>LDLFVSPLGRVEGDLDVRVTINDGVVTSAWTEAAMFRGFEIILRGKDPQAGLIVCPRICGICGGSHLYKSAYALDTAWRTHMPPNATLIRNICQACETLQSIPRYFYALFAIDLTNKNYAKSKLYDEAVRRFAPYVGTSYQPGVVLSAKPVEVYAIFGGQWPHSSFMVPGGVMSAPTLSDVTRAIAILEHWNDNWLEKQWLGCSVDRWLENKTWNDVLAWVDENESQYNSDCGFFIRYCLDVGLDKYGQGVGNYLATGTYFEPSLYENPTIEGRNAALIGRSGVFADGRYFEFDQANVTEDVTHSFYEGNRPLHPFEGETIPVNPEDGRRQGKYSWAKSPRYAVPGLGNVPLETGPLARRMA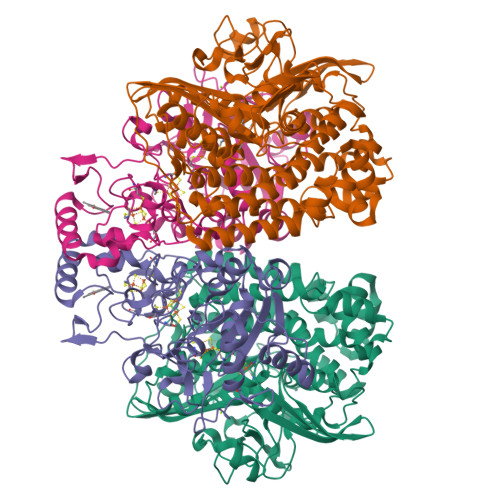ASAPDAETHQDDDPLFADIYNAIGPSVMVRQLARMHEGPKYYKWVRQWLDDLELKESFYTKPVEYAEGKGFGSTEAARGALSDWIVIEDSKIKNYQVVTPTAWNIGPRDASEVLGPIEQALVGSPIVDAEDPVELGHVARSFDSCLVCTVH[2x];>ASVLWFQGGACSGNTMSFLNADEPNVVDLIVDFGLDLLWHPSLGLELGNNAQKVFWDCAKGERPLDIFVFEGTVIEAPNGTGQMDMFAGRPMKDWVTDLAGAAQIVVAIGDCACFGGIPAMEPNPSGSTGLQFHKREKGGFLGPDFRSKMGLPVINVPGCPAHPDWITQILVALATGRAGDITLDDLHRPETFFKTFTQTGCTRVQFFEYKQSTLSFGEGTRTGCLFYEFGCRGPMTHSPCNRILWNRQSSKTRAGMPCLGCTEPEFPHFDLAPGTVFKTQKVSGMIPKEVPEGTDHLTYMGLAAAARIAAPQWSKEDMFVV[2x]>[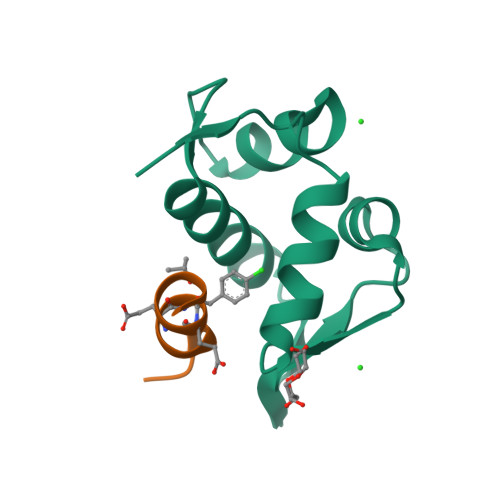2x]ETLVRPKPLLLKLLKSVGAQKDTYTMKEVLFYLGQYIMTKRLYDEKQQHIVYCSNDLLGDLFGVPSFSVKEHRKIYTMIYRNLVV;>[2x]EFWYVEXEKLLR> MGSSHHHHHHSQDPMSMTILPLELIDKCIGSNLWVIMKSEREFAGTLVGFDDYVNIVLKDVTEYDTVTGVTEKHSEMLLNGNGMCMLIPGGKPE;> MDSSPNEFLNKVIGKKVLIRLSSGVDYKGILSCLDGYMNLALERTEEYVNGKKTNVYGDAFIRGNNVLYVSALDD;> MSSLQKRPGPGNSSQPTERPRKESILDLSRYQDQRIQATFTGGRQITGILKGFDQLMNLVLDDVEEQLRNPEDGKLTGAIRKLGLVVVRGTTLVLIAPMDGSEEIPNPFVQAE

Sm and Sm-like (Lsm) proteins have been found in all three kingdoms of life: bacteria, archaea and eukaryotes. They are essential parts of ribonucleoprotein (RNP) complexes and are actively involved in various steps of RNA metabolism including pre-mRNA splicing, mRNA degradation, telomere replication, histone formation and translational control. Members of this protein family are characterized by two closely spaced, conserved Sm motifs 1 and 2, which adopt a conserved Sm fold that consists of an N-terminal α helix followed by a twisted five-stranded β sheet. A common characteristic of Sm/Lsm proteins is their tendency to form a hepta- or hexameric ring structure.

The crystal structure of SpLsm5/6/7 sub-complex was determined at a resolution of 2.3 Å by the SAD method, using phases derived from a SeMet derivative crystal. The model has been refined at the resolution of 2.3 Å to an R factor of 23.1% and Rfree of 25.4% with good stereochemistry. Several regions are disordered, namely residues 1–5 and 78–80 in Sp-Lsm5, residues 74–75 in SpLsm6, and residues 1–31, 69–77 and 101–113 in SpLsm7. Unlike SpLsm3 and SpLsm4N, the AU of the SpLsm5/6/7 crystal contains one copy of the trimeric complex. The SpLsm5/6/7 hexamer is formed by two SpLsm5/6/7 trimers related by a 2-fold symmetry. Like all Sm/Lsm oligomeric assemblies, formation of the SpLsm5/6/7 hexamer is mediated through the interaction of β4 and β5 in two neighboring Lsm subunits. The hexameric SpLsm5/6/7 ring gives three possible types of inter-subunit contacts, namely the SpLsm5/6, SpLsm5/7 and SpLsm6/7 interfaces. The structure of Lsm5/6/7 revealed that Lsm5 bridges the interaction between Lsm6 and Lsm7. The interaction of SpLsm5 with SpLsm7 is similar to that of the SpLsm5/6 interface, which involves the pairing of β5 of SpLsm5 with β4 of SpLsm7 supplemented with hydrophobic clusters and salt bridges. The observation that SpLsm5/6/7 also binds to U15 contradicts with the electrostatic potential mapping on its surface as the negatively charged helix face would prevent RNA binding.>GSMAPAGVPENTSLENIPVIVSKCREAFNDDANRDLKKRKQVLRSLLNLVEENTDEFCKAIHRDRRRHRDETVVMEILPLRNEVWHLIEHMDEYVKPVKPTMEGAAALDDCELQYEPLGVVLVIGTWNYPLLLILQPLLGALAAGNTAVIKPSELAPATAELLTKLLPKYVSSDVVGIVNGGVSETTAVLKERFDHILYTGSARVAEIVMAAAAKHLTPVTLELGGKSPVVVDDTCADNMKVVAERIMWGKIINAGQTCIAPDYVVVEKSMESVLVDALAEARKAMLGDKFLKVLKGELLVKQKQQFLEESDYPRIVNASHFQRLMEFMKGGKVAVGGEADEATLTIAPTILTNIDPTHPVMQEEIFGPILPVLTYENEKDILKIINSREKPLALYVFSNNKRFIRGVESRTSSGAVVVNDVVVHAGADGLPFGGVGRSGMGAYHGRYSFETFSHRRPVMRRGFLFSSIDTVRFPPYTTAKSRVLNSLLKPSAEVAGAVGRSVWGVAALARVVEVGYHYMRFLMAGETTPAPSSS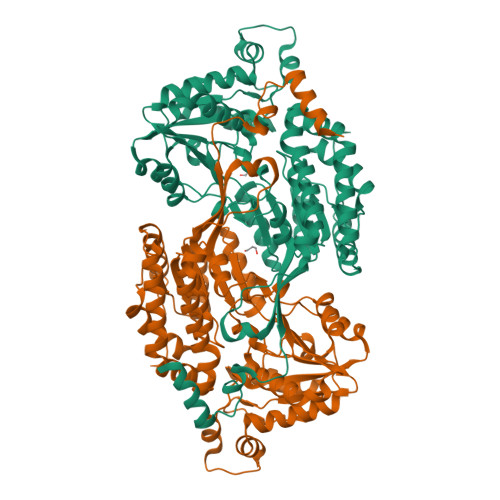EPFSKSPRSNE[2x]>AEEELPPRKVCIVGAGVSGLYIAMILDDLKIPNLTYDIFESSSRTGGRLYTHHFTDAKHDYYDIGAMRYPDIPSMKRTFNLFKRTGMPLIKYYLDGENTPQLYNNHFFAKGVVDPYMVSVANGGTVPDDVVDSVGEKLQQAFGYYKEKLAEDFDKGFDELMLVDDMTTREYLKRGGPK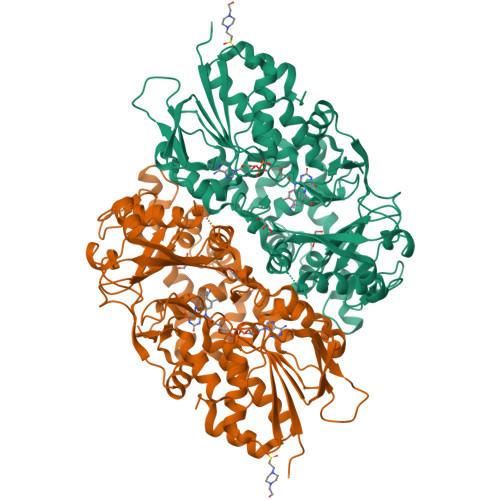GEAPKYDFFAIQWMETQNTGTNLFDQAFSESVIDSFDFDNPTKPEWYCIEGGTSLLVDAMKETLVHKVQNNKRVEAISIDLDAPDDGNMSVKIGGKDYSGYSTVFNTTALGCLDRMDLRGLNLHPTQADAIRCLHYDNSTKVALKFSYPWWIKDCGITCGGAASTDLPLRTCVYPSYNLGDTGEAVLLASYTWSQDATRIGSLVKDAPPQPPKEDELVELILQNLARLHAEHMTYEKIKEAYTGVYHAYCWANDPNVGGAFALFGPGQFSNLYPYLMRPAAGGKFHIVGEASSVHHAWIIGSLESAYTAVYQFLYKYKMWDYLRLLLERWQYGLQELETGKHGTAHLQFILGSLPKEYQVKI[2x]4-[(N-{(2E)-3-[5-chloro-2-(1H-tetrazol-1-yl)phenyl]prop-2-enoyl}-L-phenylalanyl)amino]benzoic 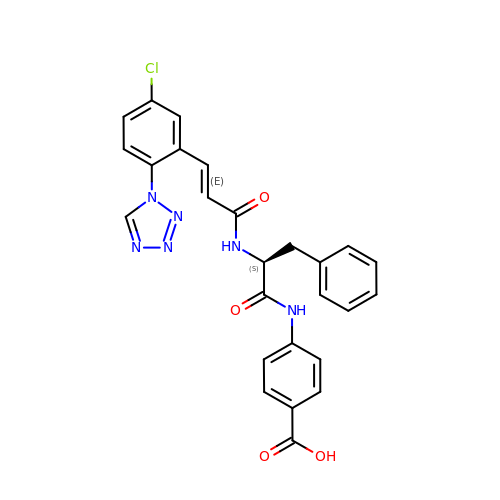acid | C26 H21 Cl N6 O4 | FMPAHDTULKAUPN-SYZXBLONSA-N> MNPPTFSPALLVVTEGDNATFTCSFSNTSESFVLNWYRMSPSGQPDKLAAFPEDRSQPGQDSRFRVTQLPNGRDFHMSVVRARRNDSGTYLCGAISL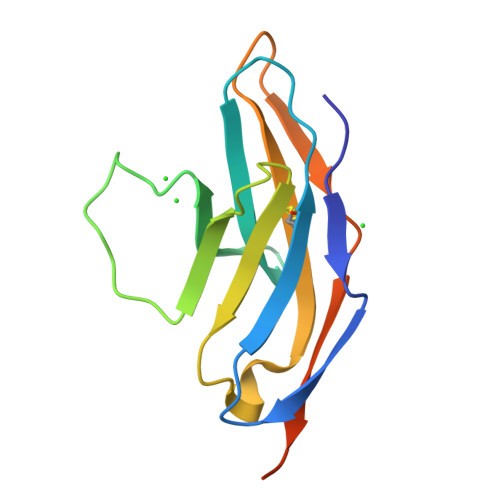APKVQIKESLRAELRVTERRAEGSWSHPQFEK> SASRKEKPKARASTPPPLNFSRASEH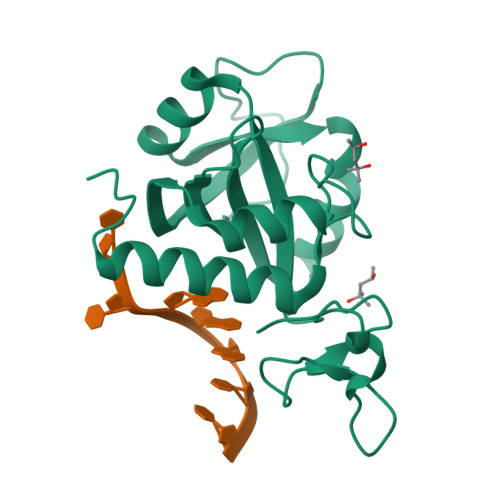RNEKGERISMINPRVVLDENGISHRSRYFIMLCDNETAIAHAKKTSIWAVKKDSSKRISDAYKKASVYFIFVAQQTYNALGYAQVVSDLNSTELPFWSDSSHAGGVRIKWIKTCNLFSAEISEIVSHMDHGSEARDGMEMMYDEGSRLCTLINYAIMKRIGRDR> MRVLITGATGGLGGAFARALKGHDLLLSGRRAGALAELAREVGARALPADLADELEAKALLEEAGPLDLLVHAVGKAGRASVREAGRDLVEEMLAAHLLTAAFVLKHARF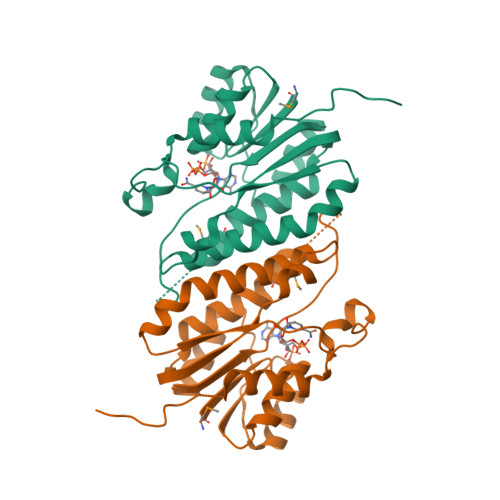QKGARAVFFGAYPRYVQVPGFAAYAAAKGALEAYLEAARKELLREGVHLVLVRLPAVATGLWAPLGGPPKGALSPEEAARKVLEGLFREPVPALLEV>MSAKAISEQTGKELLYKFICTTSAIQNRFKYARVTPDTDWARLLQDHPWLLSQNLVVKPDQLIKRRGKLGLVGVNLTLDGVKSWLKPRLGQEATVGKATGFLKNFLIEPFVPHSQAEEFYVCIYATREGDYVLFHHEGGVDVGDVDAKAQKLLVGVDEKLNPEDIKKHLLVHAPEDKKEILASFISGLFNFYEDLYFTYLEINPLVVTKDGVYVLDLAAKVDATADYICKVKWGDIEFPPPFGREAYPEEAYIADLDAKSGASLKLTLLNPKGRIWTMVAGGGASVVYSDTICDLGGVNELANYGEYSGAPSEQQTYDYAKTILSLMTREKHPDGKILIIGGSIANFTNVAATFKGIVRAIRDYQGPLKEHEVTIFVRRGGPNYQEGLRVMGEVGKTTGIPIHVFGTETHMTAIVGMALGHRPIPMGKSTTLFSRHTKAIVWGMQTRAVQGMLDFDYVCSRDEPSVAAMVYPFTGDHKQKFYWGHKEILIPVFKNMADAMRKHPEVDVLINFASLRSAYDSTMETMNYAQIRTIAIIAEGIPEALTRKLIKKADQKGVTIIGPATVGGIKPGCFKIGNTGGMLDNILASKLYRPGSVAYVSRSGGMSNELNNIISRTTDGVYEGVAIGGDRYPGSTFMDHVLRYQDTPGVKMIVVLGEIGGTEEYKICRGIKEGRLTKPIVCWCIGTCATMFSSEVQFGHAGACANQASETAVAKNQALKEAGVFVPRSFDELGEIIQSVYEDLVANGVIVPAQEVPPPTVPMDYSWARELGLIRKPASFMTSICDERGQELIYAGMPITEVFKEEMGIGGVLGLLWFQKRLPKYSCQFIEMCLMVTADHGPAVSGAHNTIICARAGKDLVSSLTSGLLTIGDRFGGALDAAAKMFSKAFDSGIIPMEFVNKMKKEGKLIMGIGHRVKSINNPDMRVQILKDYVRQHFPATPLLDYALEVEKITTSKKPNLILNVDGLIGVAFVDMLRNCGSFTREEADEYIDIGALNGIFVLGRSMGFIGHYLDQKRL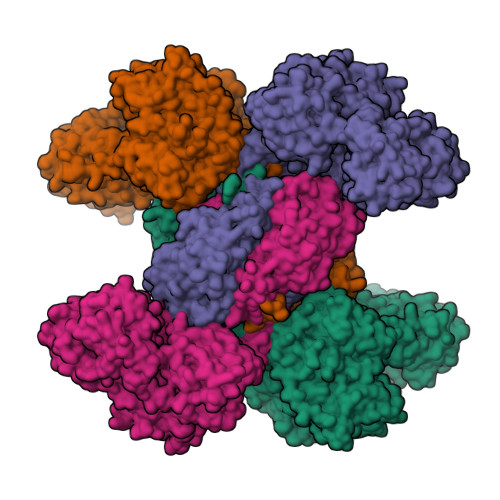KQGLYRHPWDDISYVLPEHMSMGGSHHHHHH[4x]>MAHHHHHHMTLTFNIKVIEAKDLPKVDTFGKVDPYVQIQLGNEKCKTKVI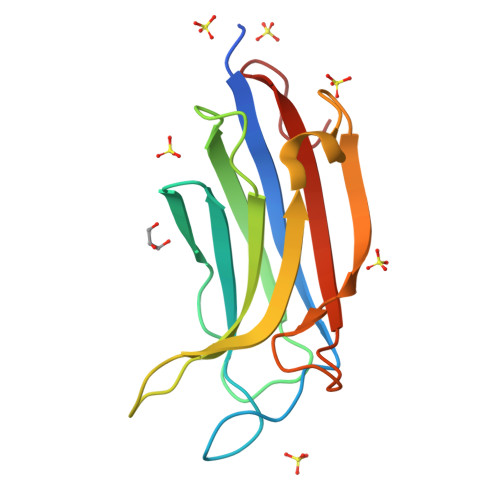KKSYNPVWNETFSIPVTNPKAPLNITVVDYDFIGSNDAFAYIHFNQQEFNVGQVVDKWYMLNSYKAGRSAGQIHLVIHLATQNMKPFE[3x]> SNAMTMKVGFIGLGIMGKPMSKNLLKAGYSLVVSDRNPEAIADVIAAGAETASTAKAIAEQCDVIITMLPNSPHVKEVALGENGIIEGAKPGTVLIDMSSIAPLASREISDALKAKGVEMLDAPVSGGEPKAIDGTLSVMVGGDKAIFDKYYDLMKAMA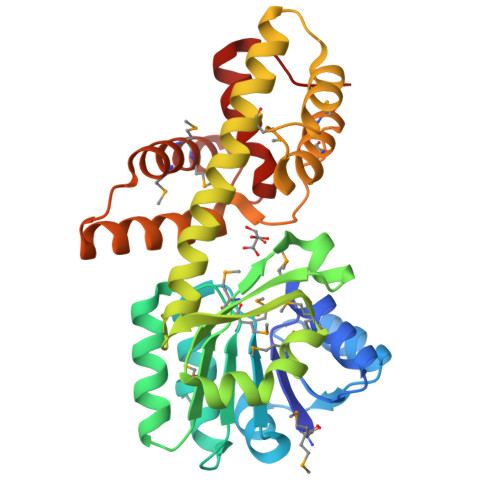GSVVHTGDIGAGNVTKLANQVIVALNIAAMSEALTLATKAGVNPDLVYQAIRGGLAGSTVLDAKAPMVMDRNFKPGFRIDLHIKDLANALDTSHGVGAQLPLTAAVMEMMQALRADGHGNDDHSALACYYEKLAKVEVTR> KYEASILTHDSSIRYLQEIYNSNNQKIVNLKEKVAQLEAQCQEPCKDTVQ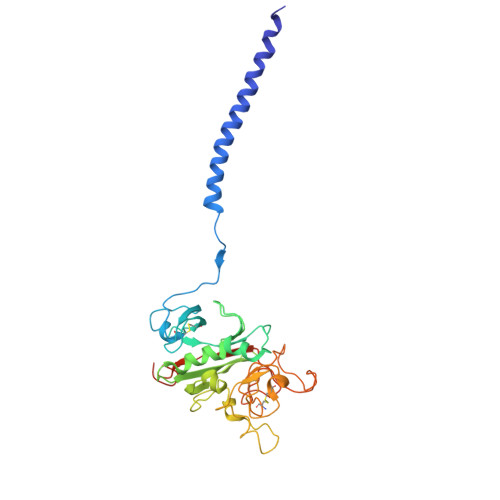IHDITGKDCQDIANKGAKQSGLYFIKPLKANQQFLVYCEIDGSGNGWTVFQKRLDGSVDFKKNWIQYKEGFGHLSPTGTTEFWLGNEKIHLISTQSAIPYALRVELEDWNGRTSTADYAMFKVGPEADKYRLTYAYFAGGDAGDAFDGFDFGDDPSDKFFTSHNGMQFSTWDNDNDKFEGNCAEQDGSGWWMNKCHAGHLNGVYYQGGTYSKASTPNGYDNGIIWATWKTRWYSMKKTTMKIIPFNRLTIGEGQQHHLGGAKQAGDV>GAMAPTPTDKHGGSDTRCPLMVKILDAVKGTPAGSVALKVSQKTADGGWTQIATGVTDATGEIHNLITE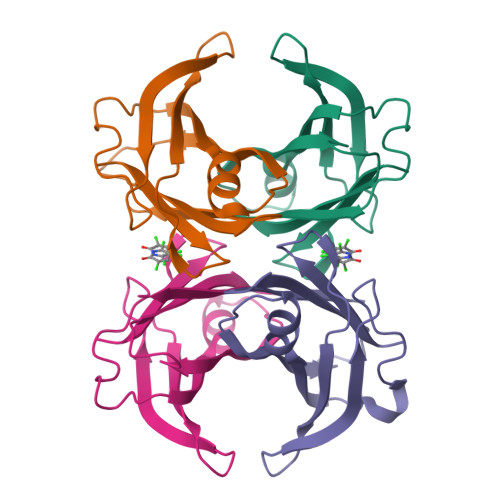QQFPAGVYRVEFDTKAYWTNQGSTPFHEVAEVVFDAHPEGHRHYTLALLLSPFSYTTTAVVSSVHE[4x]>MSNDTPFDALWQRMLARGWTPVSESRLDDWLTQAPDGVVLLSSDPKRTPEVSDNPVMIGELLHEFPDYTWQVAIADLEQSEAIGDRFGAFRFPATLVFTGGNYRGVLNGIHPWAELINLMRGLVE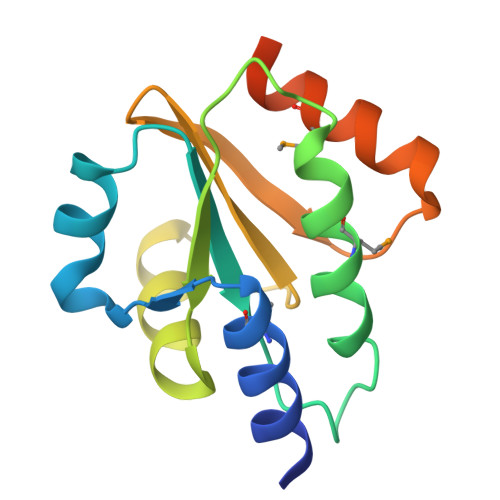PQQERASLEHHHHHH[10x]> MAALDAALYEIYDGLILYQQRLKSLEGISPELGPALDALRYDMADFAILMAQAMEEGLDSLPQSFLRKALEMIRKIQADAAALREKLAATYKGNDRAAAAQSIARKLEEMLEKAYQILRHLAAA

We use this approach with the aim of blocking the granulocyte-colony stimulating factor receptor (G-CSFR) signaling, a crucial driver of granulopoiesis, that when dysregulated can promote tumor progression and inflammatory diseases. G-CSFR is activated through ligand-induced dimerization of the ectodomains of 2 receptor subunits, which leads to the cross-phosphorylation and activation of the intracellular receptor-associated kinases. The native ligand (G-CSF) engages and dimerizes G-CSFR through 2 binding sites in a 2:2 receptor:ligand complex that juxtaposes the receptor subunits into a signaling-competent configuration. Here, we describe an approach for antagonizing cytokine receptor signaling based on designed cytokine mimics with idealized structural and biophysical properties.

Through this study, we aimed to design a series of bifaceted, designed ligands which could engage G-CSFR either in a non-signaling ternary complex, or in a 1:1 stoichiometry, outcompeting native G-CSF. By modifying designed G-CSFR binders, we engineered hyper-stable proteins that function as nanomolar signaling antagonists. X-ray crystallography showed atomic-level agreement with the experimental structure of an exemplary design. Furthermore, the most potent design blocks G-CSFR in acute myeloid leukemia cells and primary human hematopoietic stem cells. Thus, the resulting designs can be used for inhibiting or homing to G-CSFR-expressing cells.> ANVRLQHHHHHHHLESEQSEAKGFVEDANGSILFRTGYLTRDKKQGAKDTSSVAQSAIVSIESGFTPGIVGFGVGVVGDGSFKIGENKNAGNQMIPKHNDGSAYDHWARGGGSVKARFSNTTVRYGTQVLDLPVLASNTGRMVPEYFTGTLLTSHEIKNLEVVAGKFTKDQMSDQINTDADASGRGLDRAIVWGAKYKFNDNLNASYYGLDSKNALERHYANVNFKQPLANDSSLTYD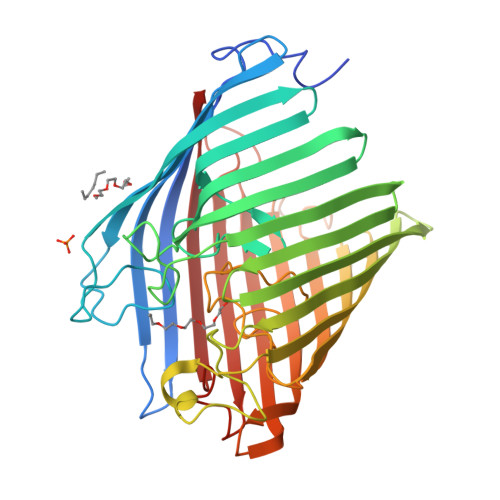FSGYHTKFDANAHTYSATGTVAPNYAADGIAGEEKTNNIWAISGTYATGPHSVMLAYQQNTGNVGYDYGQNADGFQSIYLPNSYMSDFIGNHEKSAQIQYNVDFGKLGVLPGLNWTTAFVYGWDIKVRNVTDDAQEREFFNQVKYTVQSGFAKDASLRIRNSYYRASDAYQGAYIGDTNEWRIFLDIPVKLF>GSSMVTGGMASKWDQKGMDIAYEEAALGYKEGGVPIGGCLINNKDGSVLGRGHNMRFQKGSATLHGEISTLENCGRLEGKVYKDTTLYTTLSPCDMCTGAIIMYGIPRCVVGENVNFKSKGEKYLQTRGHEVVVVDDERCKKIMKQFID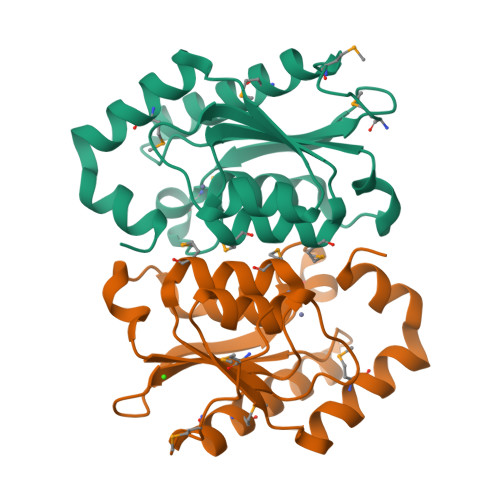ERPQDWFEDIGE[2x]>[4x]AVVEDKRAEISEIEGKLSTIQAKRIKVEKEIEAKSNELEKVSKELESSERELIAAEAQREVRGNRAAEELKRSGIGGIYGTLAEL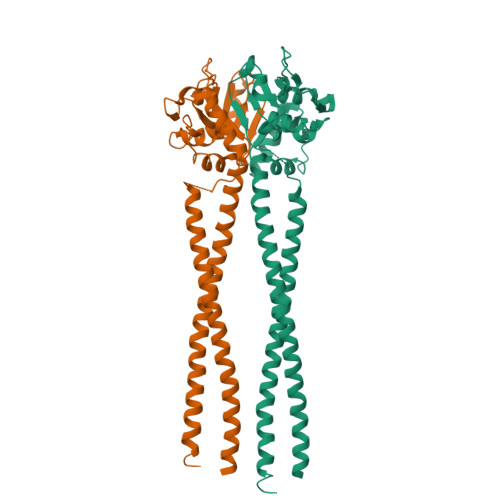IKVKDEAYALAIEVALGNRADNVVVEDELVAEKAIKYLKEHKLGRLTFLPLNKIKPKHVDSSVGLPAVDVIEYDQKIENAVKFALGDTVIVNSMEEARPHIGKVRMVTIEGELYERSGAITGGHFRARGLAVDTTKLREKVESLRRRKEALEGELNSLKIELRSLENASFELRIKLSDEKKELELASKDLN> KV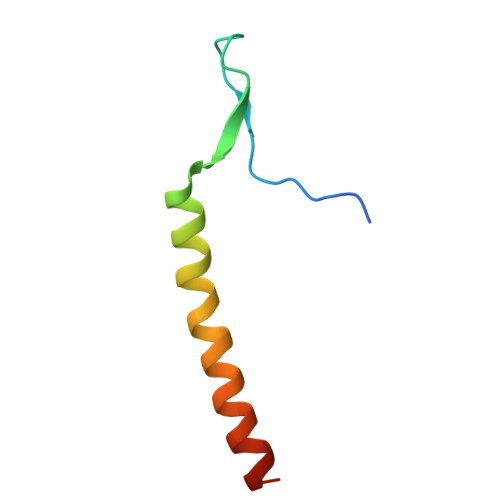ERKPPDADGCLHADPDLGVLCPTGCKLQDTLVRQERPIRKSIEDLRNTVDSVSR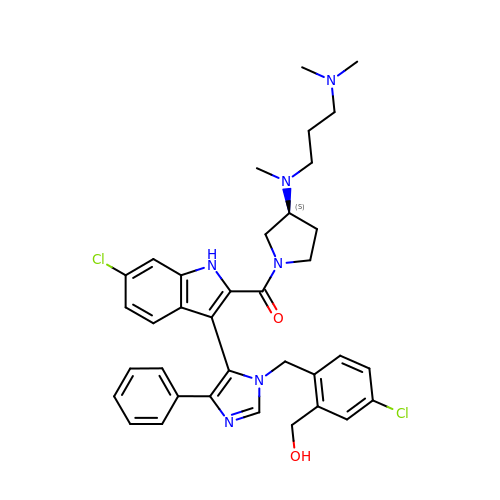[6-chloranyl-3-[3-[[4-chloranyl-2-(hydroxymethyl)phenyl]methyl]-5-phenyl-imidazol-4-yl]-1~{H}-indol-2-yl]-[(3~{S})-3-[3-(dimethylamino)propyl-methyl-amino]pyrrolidin-1-yl]methanone | C36 H40 Cl2 N6 O2 | VRHBMXYDRLEJAA-LJAQVGFWSA-N A key part of this process would have been the nonenzymatic template directed polymerization of activated RNA nucleotides. We therefore chose to use the oligoribonucleotide 5′-CCCGACUUAAGUCG-3′ which contains four locked nucleic acid (LNA) residues, denoted by italics. By obtaining crystal structures at various times after the initiation of the reaction, we were able to capture a sequence of molecular ‘snapshots’ that follow the progress of the nonenzymatic RNA polymerization reaction.

When the crystal was incubated in a solution of 2-AIpG for times over 1 hr, we began to observe the appearance of a new phosphodiester bond between the primer and the adjacent G residue. At times from 1 to 3 hr, new electron density appears between the primer 3′-hydroxyl and the 5′-phosphate of the monomer in the +1 position. The structures at 1.5 hr and 2 hr represent the average of a distribution of chemical states, and are refined as a mixture of template-bound Gp-AI-pG and the primer +1 extension product with a 2-AIpG monomer in the +2 binding site of the template. The ratio of these two states changes over time as phosphodiester bond formation proceeds to near completion by 3 hr. However, the observed decline in density for the imidazolium bridge in our current structures may also be due in part to hydrolysis of Gp-AI-pG.

> NNNGACUUAAGUCGG;> NNNGACUUAAGUCG>[2x]SAKGYVGDPSDEYYMVTFLSGIDYWKYCFEGFEDAAKAIGVTAKYTGQTDTDVSGQVAVLEQVIAQKPKGIAVTAVNSTALADTINSAIEQGISVVCFDSDSPTSNRSAYLGTGNYAAGQKAAEFLVPLVNYKGKIAVLYTVGAENSESRVQGFEDWCKQNAPEVSLVKVNDAGDTTVAADNLAAALQANDDIVGVFCVDGVAGTAGPTAVAESKKDLRVLAFDVDVTVLDKVKSGEIDGTVAQGMYNMGYWSLMMLYTEANGLSSKALPGNLDTGVVIVTKDNVDEYYPKK

Clostridium thermocellum has extensive potential in lignocellulose biorefineries as an environmentally prominent, thermophilic, cellulolytic bacterium. Previously, five putative sugar transporters, denoted A to D and L and belonging to the ABC transport systems group, were identified in the genome of C. thermocellum, and the solute-binding lipoproteins (SBP) of these ABC transporters were shown to bind different dextrins by isothermal titration calorimetry (ITC) assays. To gain insight into the structural mechanism of the transporter specificities, 11 crystal structures, both alone and in complex with appropriate saccharides, were solved for all 5 putative sugar-binding proteins, thus providing detailed specific interactions between the proteins and the corresponding saccharides. Combined genetic, biophysical, and structural studies have provided solid evidence that transporter A and transporter B are the major glucose and cellodextrin transporters, respectively, among the five potential sugar transporters in C. thermocellum.

Similar to the typical SBP fold, all of the Cbps adopted two-domain structures connected by three hinge regions, with the buried ligand-binding site between the two domains. The crystal structures of both unliganded and glucose-liganded CbpA were determined to 2.10 and 1.85 Å resolution, respectively. According to the “Venus-flytrap” mechanism, i.e., ligand binding causes a dramatic conformational change of two-domain SBPs from an open to a closed state. Hence, the structure of unliganded CbpA assumes an open conformation, while CbpA in complex with glucose adopts a closed-conformation, resulting in approximately 37° rigid-body rotation with respect to the unliganded CbpA structure. Furthermore, the binding pocket of CbpA is distinctly small for the accommodation of a monosaccharide, and no additional space appears available for the binding of larger cellodextrins in CbpA, thus explaining the functional specificity of transporter A. The ITC experiments showed that among all of the tested substrates, only CbpA binds to glucose, with a dissociation constant (KD) of 240 μM. In agreement with the ITC data, NMR titrations showed that CbpA binds glucose but not cellobiose or cellotriose.>MYMSKYVPVYTLLILIYSFNASAEWTGDNTNAYYSDEVISELHVGQIDTSPYFCIKTVKANGSGTPVVACAVSKQSIWAPSFKELLDQARYFYSTGQSVRIHVQKNIWTYPLFVNTFSANALVGLSSCSATQCFGPKLE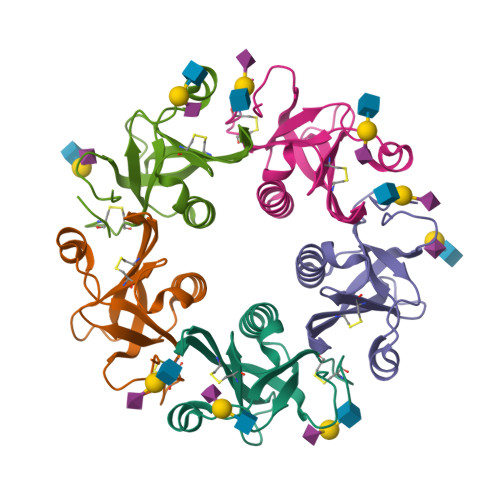HHHHHH[5x]>DLEPRFNNSSLKIEELQEALRKKEEEMKQMEERYKKYLEKAKSVIRTLDPKQNQGAAPEIQALKNQLQERDRLFHSLEKEYEKTKSQREMEEKYIVSAWYNMGMTLHKKAAEDRLASTGSGQSFLARQRQATSSRRSYPGHVQPATAR[2x];> MERMNWLSRLASRGPGHRIPQGANLQTPVMADPETCLMVFKNHWSQVVRILERQGPRAAPGGADDLSAVRNHTYQMLTLLAEDRAVPSAPTGPGPLLEFALHEDLLTRVLTWQLQWDELGDGVEERRAEQLKLFEMLVSEARQPLLRHGPVREALLTLLDACGRPVPSSPALDEGLVLLLSQLCVCVAQEPSLLEFFLQPPPEPGAAPRLLLFSRLVPFVHLEGTLGQQARDALLLLMALSAGSPTVGRYIADHSYFCPVLATGLSALYSSLPRKIEVPGDDWHCLRREDWLGVPALALFMSSLEFCNAVIQVAHPLVQKQLVDYIHNGFLVPVMGPALHKTSVEEMIASTAYLELFLRSISEPALLRTFLRFLLLHRHDTHTILDTLVARIGSNSRLCMVSLSLFRTLLNLSCEDVLLQLVLRYLVPCNHVMLSQKPAVRDVDLYGRAADKFLSLIPRCCRHHAPSPPRPEHASWARGPGSPSVDSSSVTTVPRPSTPSRLALFLRQQSLGGSESPGPAPCSPGLSASPASSPGRRPTPAEEPGELEDNYLEYLREARRGVDRCVRACRTWSAPYDGERPSPEPSPFGSRTKKRSLLPEEDRNNVGEGEEEELGRRGRAGGAGEGPGHLPPPQLNGVPGSWPEGAKKVRLVPKEGAGELLEGISEGMAGLEGFGQELRELEVALSNGGTGSESPLEPPLPLEEEEAYESFTCPPEPPGPFLSSPLRTLNQLPSQPFTGPFMAVLFAKLENMLQNSVYVNFLLTGLVAQLACHPQPLLRSFLLNTNMVFQPSVKSLLQVLGSVKNKIENFAASQEDFPALLSKAKKYLIARGKLDWAEGPAAGPAPRRSDPLVKSRRPSLGELLLRHAHSPTRARQAAQLVLQPGRDGAGLGLSGGSPGASTPVLLTRGGAPERQGEALRVKNAVYCAVIFPEFLKELAAISQAHAVTSPFLLETSEEGSGPLISGCGPLNP;> MNPFWSMSTSSVRKRSEGEEKTLTGDVKTSPPRTAPKKQLPSIPK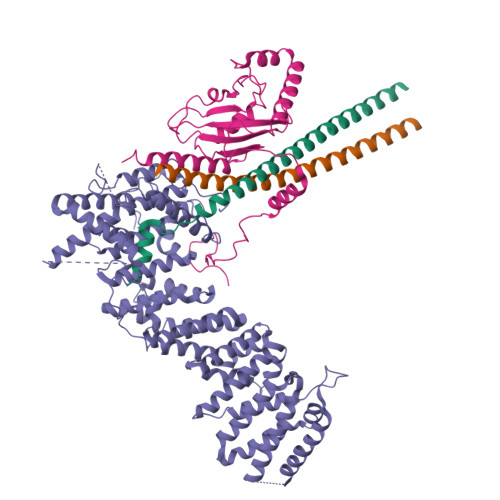NALPITKPTSPAPAAQSTNGTHASYGPFYLEYSLLAEFTLVVKQKLPGVYVQPSYRSALMWFGVIFIRHGLYQDGVFKFTVYIPDNYPDGDCPRLVFDIPVFHPLVDPTSGELDVKRAFAKWRRNHNHIWQVLMYARRVFYKIDTASPLNPEAAVLYEKDIQLFKSKVVDSVKVCTARLFDQPKIEDPYAISFSPWNPSVHDEAREKMLTQKKPEEQHNKSVHVAGLSWVKPGSVQPFSKEEKTVAT> MTC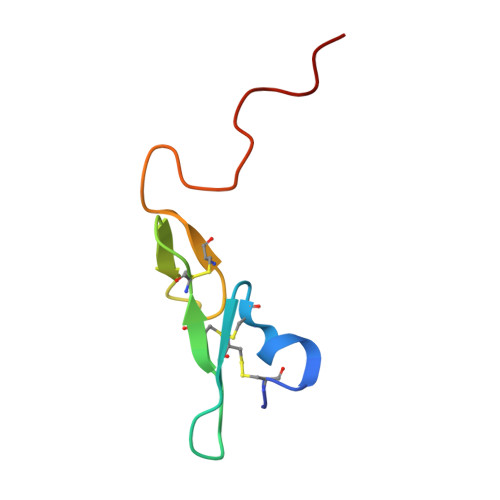NIKNGRCEQFCKNSADNKVVCSCTEGYRLAENQKSCEPAVPFPCGRVSVSQTSK> XDPASMRCHRAAHICSV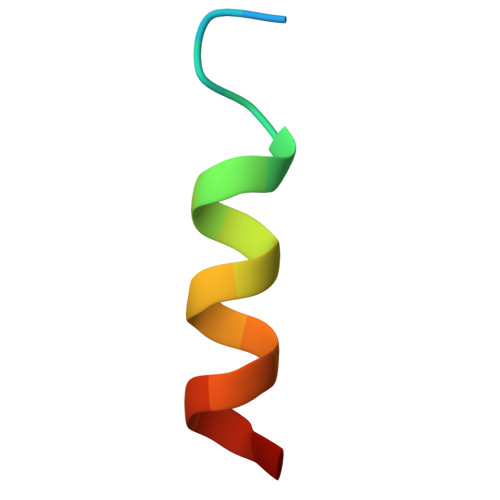LX> KEKTGQVKHKNQATHKEFSQLEKKFDARLGVYAIDTGTNQTIAYRPNERFAFASTYKALAAGVLLQQNSTKKLDEVITYTKEDLVDYSPVTEKHVDTG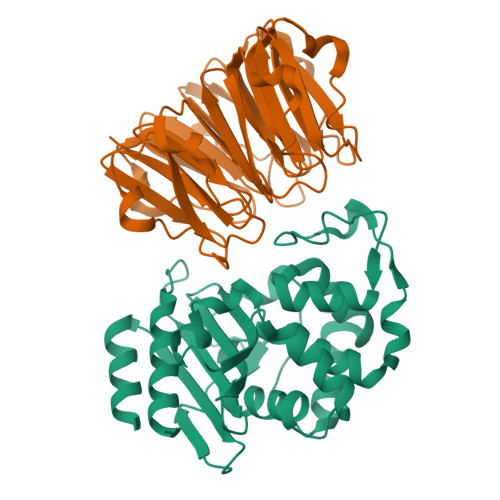MTLGEIAEAAVRYSDNTAGNILFHKIGGPKGYEKALRQMGDRVTMSDRFETELNEAIPGDIRDTSTAKAIATNLKAFTAGNALPNHKRNILTKWMKGNATGDKLIRAGVPTNWVVADKSGAGSYGTRNDIAIVWPPNRAPIIIAILSSKDEKGATYDNQLIAEAAEVIVNAFR;> ATSVVAWGGNNDWGEATVPAEAQSGVDAIAGGYFHGLALKGGKVLGWGANLNGQLTMPAATQSGVDAIAAGNYHSLALKDGEVIAWGGNEDGQTTVPAEARSGVDAIAAGAWASYALKDGKVIAWGDDSDGQTTVPAEAQSGVTALDGGVYTALAVKNGGVIAWGDNYFGQTTVPAEAQSGVDDVAGGIFHSLALKDGKVIAWGDNRYKQTTVPTEALSGVSAIASGEWYSLALKNGKVIAWGSSRTAPSSVQSGVSSIEAGPNAAYALKGGSGSGHHHHHH> GHMQIGWRREGIKYRRNELFLDVLESVNLLMSPQGQVLSAHVSGRVVMKSYLSGMPECKFGMNDKIVIEKQGKGTADETSKSGKQSIAIDDCTFHQCVRLSKFDSERSIS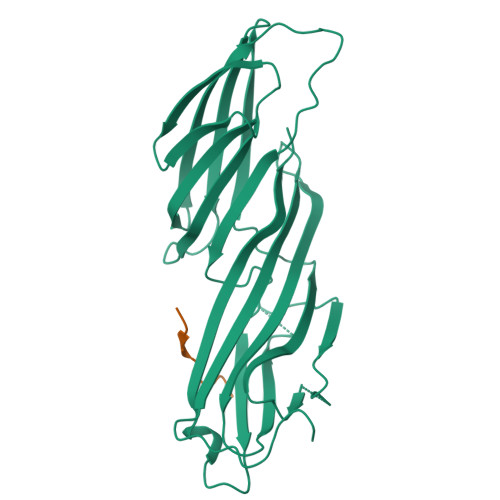FIPPDGEFELMRYRTTKDIILPFRVIPLVREVGRTKLEVKVVIKSNFKPSLLAQKIEVRIPTPLNTSGVQVICMKGKAKYKASENAIVWKIKRMAGMKESQISAEIELLPTNDKKKWARPPISMNFEVPFAPSGLKVRYLKVFEPKLNYSDHDVIKWVRYIGRSGIYETRC;> LYCYEQLNDEEEEEDEID>[2x]MMANRMILNETAWFGRGAVGALTDEVKRRGYQ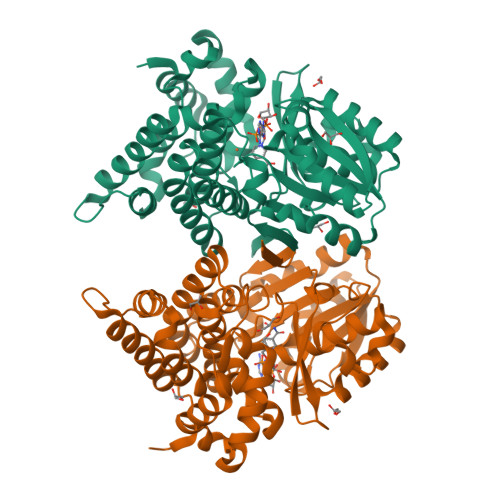KALIVTDKTLVQCGVVAKVTDKMDAAGLAWAIYDGVVPNPTITVVKEGLGVFQNSGADYLIAIGGGSPQDTCKAIGIISNNPEFADVRSLEGLSPTNKPSVPILAIPTTAGTAAEVTINYVITDEEKRRKFVCVDPHDIPQVAFIDADMMDGMPPALKAATGVDALTHAIEGYITRGAWALTDALHIKAIEIIAGALRGSVAGDKDAGEEMALGQYVAGMGISNVGLGLVHGMAHPLGAFYNTPHGVANAILLPHVMRYNADFTGEKYRDIARVMGVKVEGMSLEEARNAAVEAVFALNRDVGIPPHLRDVGVRKEDIPALAQAALDDVCTGGNPREATLEDIVELYHTAWTSHHHHH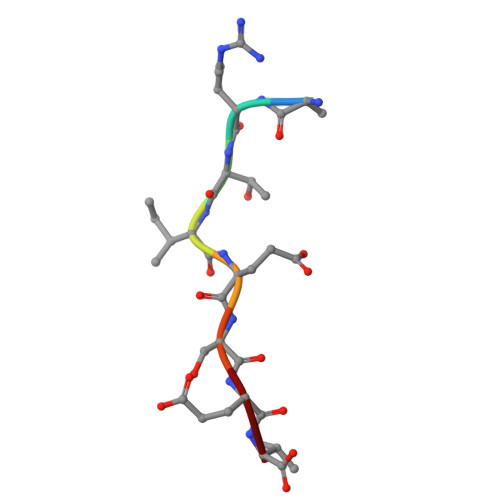> ARTIESEV>[2x]GTKQEKT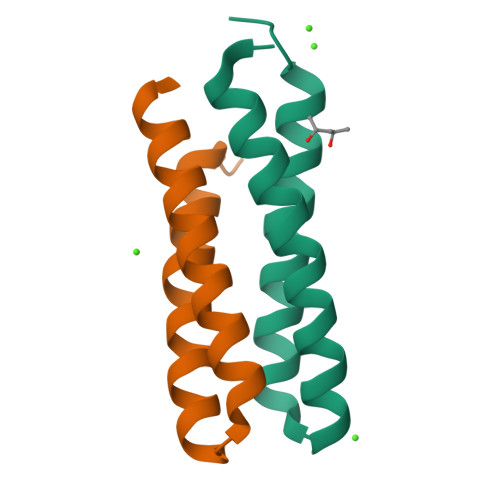ILNMARFIRSQALTILEKANELDADEIADIAESIHDHADEIYRSALARFGDDGENL> WSHPQFEKMQLNKEVLKGYIDILIVSILEKKDCYGYEIAKQVRERSEFELKEGTMYLALKRMESKNLIKSYYSNEQSSGGRRKYYNLTNEGKDFLEIKKQEWRFIKKVMNQFLGEVD

We examined the structure and function of a gene product with the locus tag CDR20291_0991 (cdPadR1) as part of our broader goal aimed at elucidating transcription regulatory mechanisms involved in virulence and antibiotic resistance of the recently emergent hypervirulent C. difficile strain R20291. cdPadR1 is genomically positioned near genes that are involved in stress response and virulence. We have determined the 1.9 Å resolution crystal structure of cdPadR1, which revealed that it is in the PadR-s2 subfamily of PadR transcriptional regulators with other structurally and functionally characterized PadR-like regulators from B. cereus (bcPadR1 and bcPadR2) and L. lactis (LmrR). We also demonstrate cdPadR1 binding to its own gene promoter in a manner conducive to autoregulation. Additionally, we show that cdPadR1 binds the promoters of three additional regulatory signaling proteins and that a cdPadR1 binding motif is present upstream of 100 genes in C. difficile R20291.

One molecule of cdPadR1 was present in the asymmetric unit and consists of an N-terminal winged helix-turn-helix (wHTH) domain (residues 6–80) and a single α-helical C-terminal domain (residues 81–106). The dimeric state of cdPadR1 is retained in solution as determined by size exclusion chromatography. The recognition helices (α3/ α3’) are positioned ~34 Å apart in cdPadR1, which is consistent with symmetrical binding to two “half-sites” comprised of inverted repeats ~10 bp apart; it is important to note that this distance does not account for DNA secondary structure. Dimerization of cdPadR1 buries approximately 1100 Å2 solvent-accessible surface area (16 %) of the approximately 7000 Å2 total solvent-accessible area per subunit. Residues on helices α1, α2, and α4 that interact to form the cdPadR1 dimer interface are conserved across structural homologues. Helix α4 and α4′of cdPadR1 bend toward each other and interact via a coiled-coil, whereas α4 and α4′ of LmrR do not display a significant bending towards each other at the C-terminus (red). In addition, LmrR contains fewer residues involved in dimerization at the C-terminus of the helix than cdPadR1 and bcPadRs. cdPadR1, like bcPadRs and ctPadR, has a closed dimeric interface, unlike the hydrophobic pore wherein aromatic drug-interaction occurs in LmrR. The P-P, I-I, and I-P distances between cdPadR1 W94 and W94′ are 5.4 Å, 9.2 Å, and 7.4 Å, respectively. The P-P distance is ~2 Å greater for the apo-LmrR (P-P = 6.9 Å), LmrR-H33342 (P-P = 7.2 Å), and LmrR-daunomycin (P-P = 7.4 Å) structures when compared to the distance between phenol centroids in cdPadR1. The lack of a drug-binding pocket in cdPadR1 suggests that any differential expression of the CD630 homologue (CD630_1154) during Mtz exposure would, most likely, be due to a regulatory cascade effect rather than direct interaction of cdPadR1 with Mtz.> MSTYEGRWKTVKVEIEDGIAFVILNRPEKRNAMSPTLNREMIDVLETLEQDPAAGVLVLTGAGEAWTAGMDLKEYFREVDAGPEILQEKIRREASQWQWKLLRM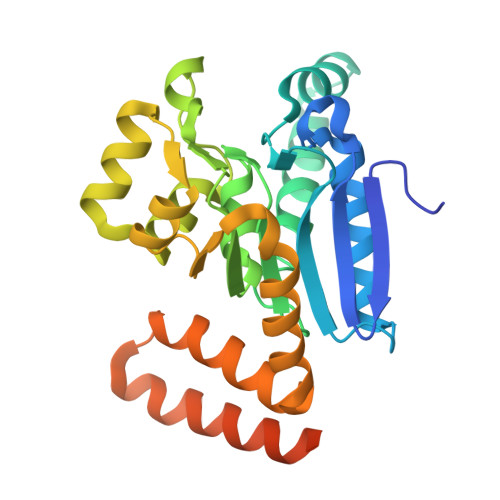YAKPTIAMVNGWCFGGGFSPLVACDLAICADEATFGLSEINWGIPPGNLVSKAMADTVGHRQSLYYIMTGKTFGGQKAAEMGLVNESVPLAQLREVTIELARNLLEKNPVVLRAAKHGFKRCRELTWEQNEDYLYAKLDQSRLLDTEGGREQGMKQFLDDKSIKPGLQAYKR> AAAADWKSRSIYQLVTDRFGRSDGSTSACGDLSNYCGGDYKGIQNQLDYIAGMGFDAIWISPIPENTDGGYHGYWAKDFEKLNTNFGSADDLKALVTAAHGKGMYVMLDVVANHAGPASGGDYSGFTFSSASNYHPQCTIDYDNQTSVEQCWVADDLPDINTEDDTIVSKLHSIVSDWVTTYDFDGIRIDTVKHIRKDFWSGYEEAAGVFATGEVFDGDAAYVGPYQDQLSSLINYPLYYAIRDVFSAGSGFSRISDMLSTIKSNFKDPSVLTTFVDNQDNARFLSVKSDMSLYKNALAFTIL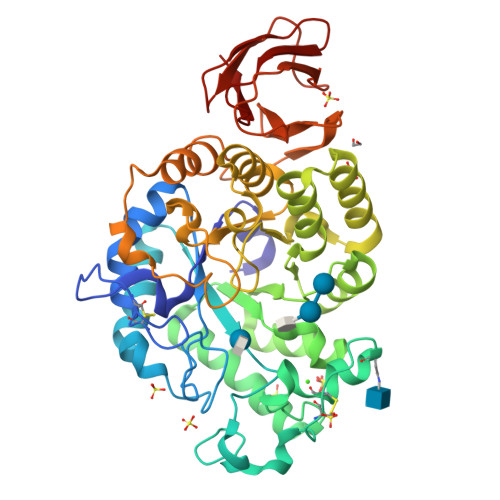TEGIPVVYYGTEQGFKGGDDPKNREVLWTSNYDTSSDLYKFIKIVNNDVRQKSDKTVTLDVDVGTNTYAFTHGKNLIVVNNYGSGSTESVTVKVGDSVADGTKLVDAVSNITATVSGGSITFSLKDGLPALFVPSS>[2x]GMDKLVKYQELVKKLLTNYASDDVSDQDVEVQLILDTERNHYQWM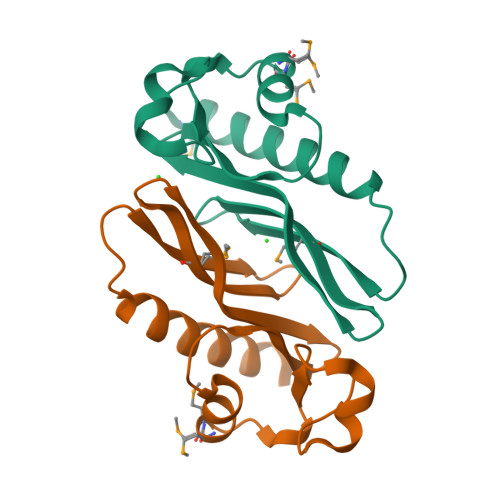NVGWQGLNRIYRCVIHFDIKDGKIWLQQNLTDRNPAEELVMMGVPREDIVLGLQAPYKRQYTDYGVA> SEVPMGVEIVEAPAVWRASAKGAGQIIGVIDTGCQVDHPDLAERIIGGVNLTTDYGGDETNFSDNNGHGTHVAGTVAAAETGSGVVGVAPKADLFIIKALSGDG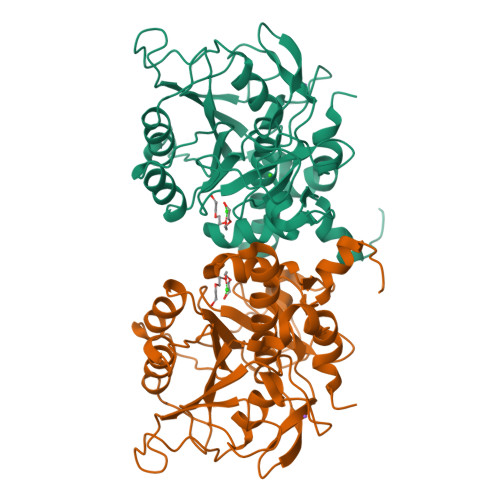SGEMGWIAKAIRYAVDWRGPKGEQMRIITMSLGGPTDSEELHDAVKYAVSNNVSVVCAAGNEGDGREDTNEFAYPAAYNEVIAVGAVDFDLRLSDFTNTNEEIDIVAPGVGIKSTYLDSGYAELSGTAMAAPHVAGALALIINLAEDAFKRSLSETEIYAQLVRRATPIGFTAQAEGNGFLTLDLVERITGQFTEKGKKLEHHHHHH>[5x]SNAMIIRPEQHWFLRLFDWHGSVLSKIIFRLLLNVLMSIIAIISYQWYEQLGIHLTVAPFSLLGIAIAIFLGFRNSASYSRFVEARNLWGTVLIAERTLVRQLRNILPAEHDAHRRIVSYLVAFSWSLKHQLRKTDPTADLRRLLPEERVTEILASSMPTNRILLLAGNEIGQLREAAKLSDITYGLMDNKLDELAHVLGGCERLATTPVPFAYTLILQRTVYLFCTLLPFALVGDLHYMTPFVSVFISYTFLSWDSLAEELEDPFGTAANDLPLNAMCNTIERNLLDMTGQHPLPE

Human bestrophin1 (hBest1) is a Ca2+-activated Cl− channel essential for Cl− transport in retinal pigment epithelium (RPE). Although the structure of hBest1 is still unsolved, two Best1 homolog structures, one from bacteria Klebsiella pneumoniae (KpBest) and the other from chicken (cBest1), have been previously reported. Overall, the channel is a pentameric assembly with a single ion-conducting pathway, which varies in diameter along its length and is constrained at two narrow points: a “neck” contributed by three residues (I62/I66/F70 in KpBest and I76/F80/F84 in hBest1/cBest1) on a transmembrane helix, and an “aperture” formed by a single residue (I180 in KpBest1, I205 in hBest1, and V205 in cBest1) on a cytosolic helix. Here, by electrophysiological and structural analyses, we show that the neck and aperture in hBest1 are both indispensable Ca2+-dependent gates, and their dysregulated opening by rationally designed or patient-derived mutations causes Ca2+-independent leak and elevates Ca2+-dependent channel activity.

Twelve identical residues shared between KpBest and hBest1 on the loop structures within the channel core transmembrane regions were identified as the subjects of alanine substitution, as we reasoned that replacing conserved residues on the (relatively flexible) loops, rather than substitution on the rigid helices, are more likely to be informative without disrupting the overall channel structure. Alanine substitution mutants for each of the 12 residues were generated in KpBest and hBest1 and subjected to crystallography and patch clamp, respectively. All 12 KpBest mutants were purified with a size exclusion profile indistinguishable from the WT, suggesting that the overall integrity of the channel is still retained after alanine substitution. Eleven of the 12 KpBest mutant structures were solved, while 10 of the 12 hBest1 mutants displayed altered channel function.> MPNSEPASLLELFNSIATQGELVRSLKAGNASKDEIDSAVKMLVSLKMSYKAAAGEDYKADCPPGNPAPTSNHGPDATEAEEDFVDPWTVQTSSAKGIDYDKLIVRFGSSKIDKELINRIERATGQRPHHFLRRGIFFSHRDMNQVLDAYENKKPFYLYTGRGPSSEAMHVGHLIPFIFTKWLQDVFNVPLVIQMTDDEKYLWKDLTLDQAYSYA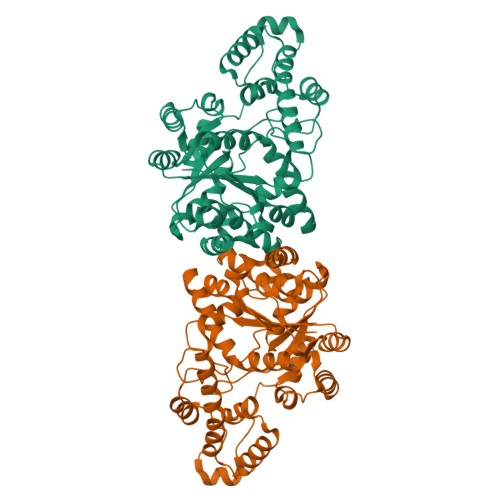VENAKDIIACGFDINKTFIFSDLDYMGMSSGFYKNVVKIQKHVTFNQVKGIFGFTDSDCIGKISFPAIQAAPSFSNSFPQIFRDRTDIQCLIPCAIDQDPYFRMTRDVAPRIGYPKPALLHSTFFPALQGAQTKMSASDPNSSIFLTDTAKQIKTKVNKHAFSGGRDTIEEHRQFGGNCDVDVSFMYLTFFLEDDDKLEQIRKDYTSGAMLTGELKKALIEVLQPLIAEHQARRKEVTDEIVKEFMTPRKLSFDFQHHHHHH Here, the first crystal structures from PF02663 are described, representing two bacterial and one archaeal species: B8FYU2_DESHY from the anaerobic dehalogenating bacterium Desulfito­bacterium hafniense DCB-2, Q2LQ23_SYNAS from the syntrophic bacterium Syntrophus aciditrophicus SB and Q9HJ63_THEAC from the thermoacidophilic archaeon Thermoplasma acidophilum. Two of these proteins, Q9HJ63_THEAC and Q2LQ23_SYNAS, contain two domains: an N-terminal thioredoxin-like α+β core domain (NTD) consisting of a five-stranded, mixed β-sheet flanked by several α-helices and a C-terminal zinc-finger domain (CTD). The proximity of fmdE to genes encoding the catalytic subunits suggests a role in methanogenesis for proteins in PF02663. Individual proteins within this family display differences in domain architectures, metal-ion binding propensities and dimer interactions.

The final model includes one protein molecule (residues 1–190), one chloride anion, one Zn atom and 42 water molecules in the asymmetric unit. The total β-sheet, α-helical and 310-helical contents are 18, 56 and 4.9%, respectively. Q2LQ23_SYNAS displays a similar architecture to Q2HJ63_THEAC, with a larger NTD (residues 1–154) and a smaller, treble-clef zinc-finger domain CTD coupled together through a nine-residue linker (residues 155–163). The linkers in Q9HJ63_THEAC and Q2LQ23_SYNAS separate the NTD and CTD domains so that the closest edges of the two domains are ∼20 Å apart. Two significant structural differences between Q9HJ63_THEAC and Q2LQ23_SYNAS involve their metal binding. First, zinc is bound to the putative active site on the NTD of Q9HJ63_THEAC, but is absent from the NTD of Q2LQ23_SYNAS. Second, whereas the structure of the CTD of Q2LQ23_SYNAS shows four Cys side chains within coordination distance of the Zn atom, the structure of Q9HJ63_THEAC is atypical for a treble-cleft zinc finger in that three Cys side chains and an Asp side chain are within coordination distance of the zinc. In Q2LQ23_SYNAS no zinc is bound to the NTD. The chloride is bound near the end of the central β-sheet facing towards the extended stretch of polypeptide connecting the NTD and the CTD on the symmetry-related subunit. The overall fold of the zinc-finger domains of Q9HJ63_THEAC (residues 171–201) and Q2LQ23_SYNAS (residues 162–190) are similar, with an r.m.s.d. of 1.1 Å for 24 superposed Cα atoms.

> GMTARNILSYSYEEYVEKITAFHGYPAPGVLIGGFMVDLAVKNLPEGILYDAICETRTCLPDAVQLLTPCTFGNGWLTVLPMGLFAVSLYDKFTGEGVRVFLDVEKMGPWQEIRNWFLKLKTKKEQDSERLFKEIREAGPDILELRNVKLKPGFLEKKHKGKIVLCPQCREAYPAQDGELCLSCQGGSPYL>[12x]MDAEGLALLLPPVTLAALVDSWLREDCPGLNYAALVSGAGPSQAALWAKSPGVLAGQPFFDAIFTQLNCQVSWFLPEGSKLVPVARVAEVRGPAHCLLLGERVALNTLARCSGIASAAAAAVEAARGAGWTGHVAGTRKTTPGFRLV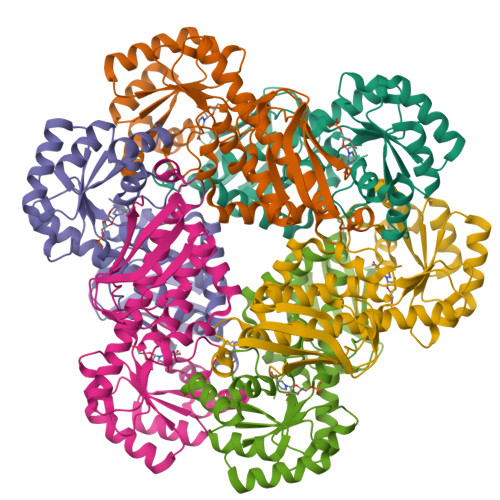EKYGLLVGGAASHRYDLGGLVMVKDNHVVAAGGVEKAVRAARQAADFALKVEVECSSLQEAVQAAEAGADLVLLDNFKPEELHPTATVLKAQFPSVAVEASGGITLDNLPQFCGPHIDVISMGMLTQAAPALDFSLKLFAKEVAPVPKIHLEHHHHHH>GAMGSFN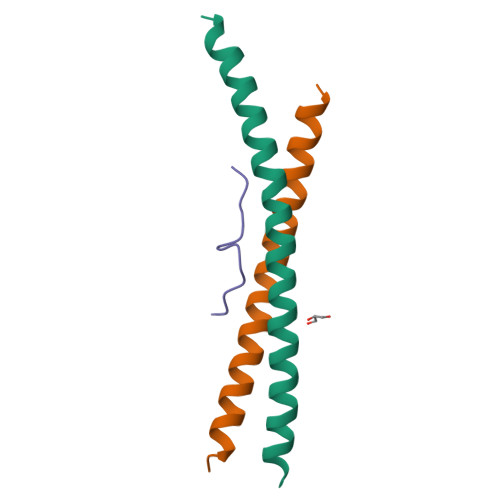SSINNIHEMEIQLKDALEKNQQWLVYDQQREVYVKGLLAKIFELEKKTETAAHSLP[8x];>DLAVGPPSLNYIPP[4x]>[2x]MGSDKIHHHHHHMNVLALDTSQRIRIGLRKGEDLFEISYTGEKKHAEILPVVVKKLLDELDLKVKDLDVVGVGIGPGGLTGLRVGIATVVGLVSPYDIPVAPLNSFEMTAKSCPADGVVLVARRARKGYHYCAVYLKDKGLNPLKEPSVVSDEELEEITKEFSPKIVLKDDLLISPAVLVEESERLFREKKTIHYYEIEPLYLQKSIAELNWEKKKRG

YeaZ is involved in a protein network that is essential for bacteria. yeaZ is an essential gene in many bacteria, such as Escherichia coli (yeaZ), Salmonella typhimurium LT2 (yeaZ), Bacillus subtilis (ydiC), Streptococcus pneumoniae (spr0129), Pseudo­monas aeruginosa (PA14_16710) and Francisella novicida (FTN_1148). A recent study further demonstrated that E. coli YeaZ can interact with either YgjD or YjeE, with YgjD as the preferred partner, suggesting that YeaZ is part of a protein network that may be involved in DNA metabolism and cell division. TmYeaZ belongs to the actin-like ATPase superfamily, which typically contains a duplication of ribonuclease H-like domains.

The crystal structure of TmYeaZ was determined in space group C222 at 2.5 Å resolution using the MAD method. TmYeaZ is composed of nine β-strands (β1–­β9), six α-helices (α1–α6) and four 310-helices (η1–η4). In TmYeaZ, the first ribonuclease H-like domain is composed from both the N-terminus (residues 1–100) and the C-terminus (residues 160–193) of the protein. Compared with the other two YeaZs, TmYeaZ lacks the 20-residue αβ insertion between β9 and α5 in the second domain. As a monomer of His-tagged SeMet-TmYeaZ would have a calculated molecular weight of 24 404 Da, it is likely that TmYeaZ exists as a dimer in solution. Based on its structure, TmYeaZ by itself is not likely to be an ATPase owing to the absence of a clearly defined ATP-binding site. The most prominent common feature of these proteins is the prevalence of the sequence motif GPGXXTGXR located at the N-­terminus of a helix (α2 of TmYeaZ). Other conserved residues of the YeaZ homologs that are clustered around this motif include residues from the N-terminus of α1 (Lys32 and His33), the C-terminus of β1 (Asp7 and Thr8), the C-terminal portion of β6 (Arg112, Ala113 and Arg114), β7 (Tyr119) and the C-­terminus of α6 (Pro188, Tyr190 and Gln192). We speculate that part of or the entire conserved surface is involved in mediating protein–protein interactions between YeaZ and YgjD (TM0145) or YjeE (TM1632) in T. maritima. As the UNL is close to the conserved surface identified above, it may have functional implications; an alternative explanation that cannot be ruled out at present is that it is a crystallization artifact.>AHRDSGTAKSGLYVEKVSGLRKDFIKGVDVSSIIALEESGVAFYNESGKKQDIFKTLKEAGVNYVRVRIWNDPYDANGNGYGGGNNDLEKAIQIGKRATANGMKLLADFHYSDFWADPAKQKAPKAWANLNFEDKKTALYQYTKQSLKAMKAAGIDIGMVQVGNETNGGLAGETDWAKMSQLFNAGSQAVRETDSNILVALHFTNPETSGRYAWIAETLHRHHVDYDVFASSYYPFWHGTLKNLTSVLTSVADTYGKKVMVAETSYTYTAEDGDGHGNTAPKNGQTLNNPVTVQGQANAVRDVIQAVSDVGEAGIGVFYWEPAWIPVGPAHRLEKNKALWETYGSGWATSYAAEYDPED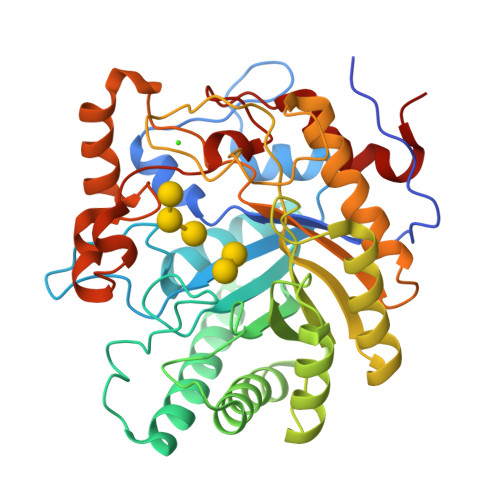AGKWFGGSAVDNQALFDFKGRPLPSLHVFQYVDTGTPFKN[2x]> MENDPNLFVALYDFVASGDNTLSI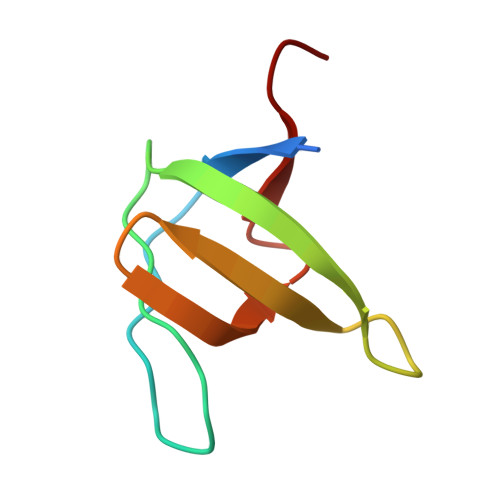TKGEKLRVLGYNHNGEWCEAQTKNGQGWVPSQYITPVNS>[2x]GSGSPLAQQIKNIHSFIHQAKA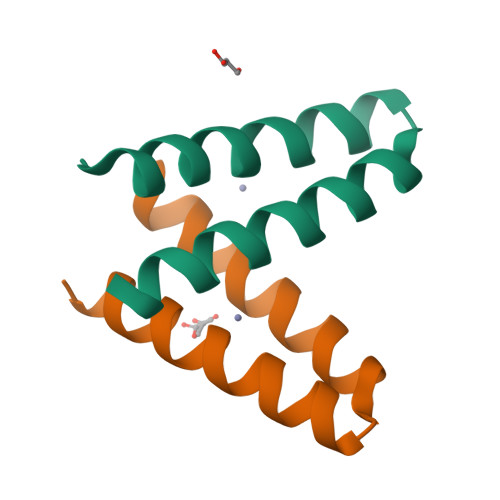AGRMDEVRTLQENLEQLMHEYFQQSD> NYIVPGEYRVAEGEIEINAGREK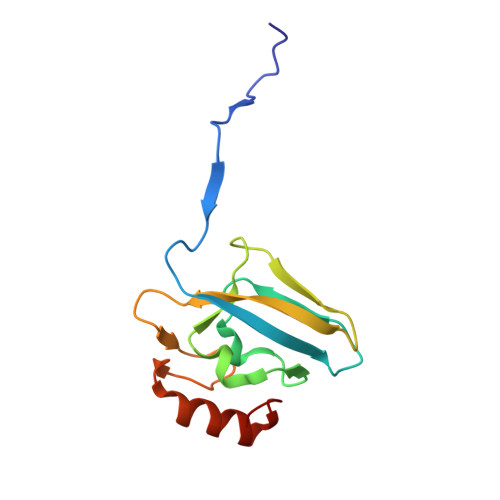TTIRVSNTGDRPIQVGSHIHFVEVNKELLFDRAEGIGRRLNIPSGTAARFEPGEEMEVELTELGGNREVFGISDLTNGSVDNKELILQRAKELGYKGVE> GAMGRSVYELDCIPLWGTVSIQGNRSEMEDAFAVSPHFLKLPIKMLMGDHEGMSPSLTHLTGHFFGVYDGHGGHKVADYCRDRLHFALAEEIERIKDELCKRNTGEGRQVQWDKVFTSCFLTVDGEIEGKIGRAVVGSSDKVLEAVASETVGSTAVVALVC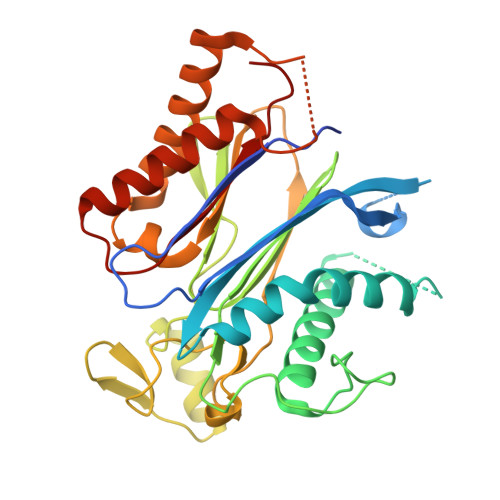SSHIVVSNCGDSRAVLFRGKEAMPLSVDHKPDREDEYARIENAGGKVIQWQGARVFGVLAMSRSIGDRYLKPYVIPEPEVTFMPRSREDECLILASDGLWDVMNNQEVCEIARRRILMWHKKNGAPPLAERGKGIDPACQAAADYLSMLALQKGSKDNISIIVIDLKAQR>GSDILQGTDYSKIQIPKQEKWQRSMSSVTEDKERQWVDDFPLHRSACEGDSELLSRLLSERFSVNQLDSDHWAPIHYACWYGKVEATRILLEKGKCNPNLLNGQLSSPLHFAAGGGHAEIVQILLNHPETDRHITDQQGRSPLNICEENKQNNWEEAAKLLKEAINKPYEKVRIYRMDGSYRSVELKHGNNTTVQQIMEGMRLSQETQQYFTIWICSENLSLQLKPYHKPLQHVRDWPEILAELTNLDPQRETPQLFL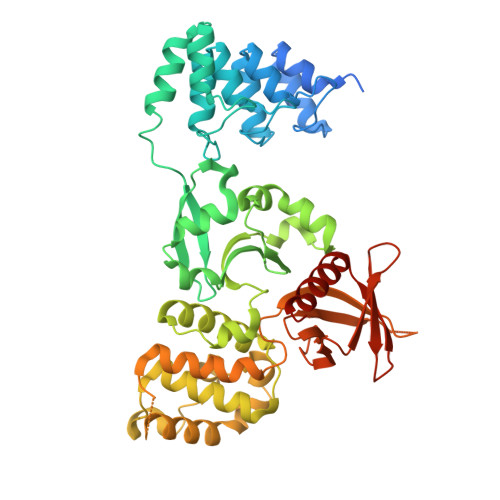RRDVRLPLEVEKQIEDPLAILILFDEARYNLLKGFYTAPDAKLITLASLLLQIVYGNYESKKHKQGFLNEENLKSIVPVTKLKSKAPHWTNRILHEYKNLSTSEGVSKEMHHLQRMFLQNCWEIPTYGAAFFTGQIFTKASPSNHKVIPVYVGVNIKGLHLLNMETKALLISLKYGCFMWQLGDTDTCFQIHSMENKMSFIVHTKQAGLVVKLLMKLNGQLMPTERNS[3x]>[6x]MRGSHHHHHHGSREGRFVPGTPRHGFVEGTEGALPKQADVVVVGAGILGIMTAINLVERGLSVVIVEKGNIAGEQSSRFYGQAISYKMPDETFLLHHLGKHRWREMNAKVGIDTTYRTQGRVEVPLDEEDLVNVRKWIDERSKNVGSDIPFKTRIIEGAELNQRLRGATTDWKIAGFEEDSGSFDPEV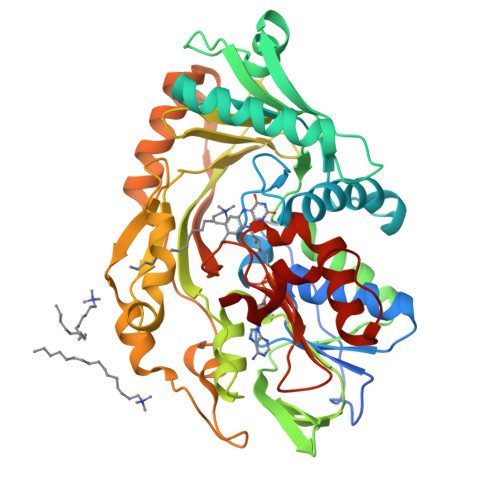ATFVMAEYAKKMGVRIYTQCAARGLETQAGVISDVVTEKGAIKTSQVVVAGGVWSRLFMQNLNVDVPTLPAYQSQQLISGSPTAPGGNVALPGGIFFREQADGTYATSPRVIVAPVVKESFTYGYKYLPLLALPDFPVHISLNEQLINSFMQSTHWNLDEVSPFEQFRNMTALPDLPELNASLEKLKAEFPAFKESKLIDQWSGAMAIAPDENPIISEVKEYPGLVINTATGWGMTESPVSAELTADLLLGKKPVLDPKPFSLYRF> MGINGQQYYIDPTTGQPRKNFLLQNGNDWIYFDKDTGAGTNALKLQFDKGTISADEQYRRGNEAYSYDDKSIENVNGYLTADTWYRPKQILKDGTTWTDSKETDMRPILMVWWPNTVTQAYYLNYMKQYGNLLPASLPSFSTDADSAELNHYSELVQQNIEKRISETGSTDWLRTLMHEFVTKNSMWNKDSENVDYGGLQLQGGFLKYVNSDLTKYANSDWRLMNRTATNIDGKNYGGAEFLLANDIDNSNPVVQAEELNWLYYLMNFGTITGNNPEANFDGIRVDAVDNVDVDLLSIARDYFNAAYNMEQSDASANKHINILEDWGWDDPAYVNKIGNPQLTMDDRLRNAIMDTLSGAPDKNQALNKLITQSLVNRANDNTENAVIPSYNFVRAHDSNAQDQIRQAIQAATGKPYGEFNLDDEKKGMEAYINDQNSTNKKWNLYNMPSAYTILLTNKDSVPRVYYGDLYQDGGQYMEHKTRYFDTITNLLKTRVKYVAGGQTMSVDKNGILTNVRFGKGAMNATDTGTDETRTEGIGVVISNNTNLKLNDGESVVLHMGAAHKNQKYRAVILTTEDGVKNYTNDTDAPVAYTDANGDLHFTNTNLDGQQYTAVRGYANPDVTGYLAVWVPAGAADDQDARTAPSDEAHTTKTAYRSNAALDSNVIYEGFSNFIYWPTTESERTNVRIAQNADLFKSWGITTFELAPQYNSSKDGTFLDSIIDNGYAFTDRYDLGMSTPNKYGSDEDLRNALQALHKAGLQAIADWVPDQIYNLPGKEAVTVT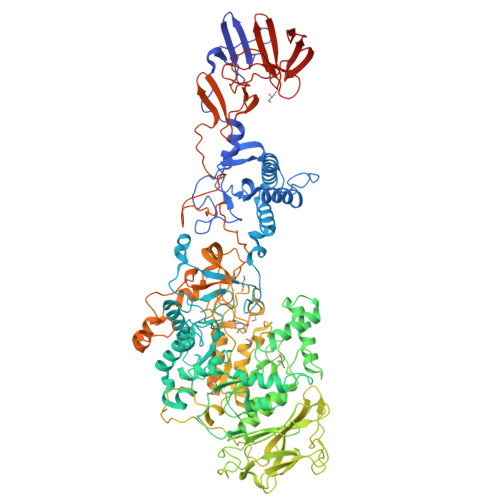RSDDHGTTWEVSPIKNVVYITNTIGGGEYQKKYGGEFLDTLQKEYPQLFSQVYPVTQTTIDPSVKIKEWSAKYFNGTNILHRGAGYVLRSNDGKYYNLGTSTQQFLPSQLSVQDNEGYGFVKEGNNYHYYDENKQMVKDAFIQDSVGNWYYLDKNGNMVANQSPVEISSNGASGTYLFLNNGTSFRSGLVKTDAGTYYYDGDGRMVRNQTVSDGAMTYVLDENGKLVSESFDSSATEAHPLKPGDLNGQKHHHHHH>[10x]SVDREEMIERFANFLREYTDEDGNPVYRGKITDLLTITPKRSVAIDWMHLNSFDSELAHEVIENPEEGISAAEDAIQIVLREDFQREDVGKIHARFYNLPETLMVKDIGAEHINKLIQVEGIVTRVGEIKPFVSVAVFVCKDCGHEMIVPQKPYESLEKVKKCEQCGSKNIELDVNKSSAVNFQSFRIQDRPETLKGGEMPRFIDGILLDDIVDVALPGDRVIVTGILRVVLEKREKTPIFRKILEVNHIEPVSKEI

The Minichromosome Maintenance (MCM) complex forms an essential hexameric-ring helicase that unwinds DNA at the replication fork (1–3). MCM proteins have three conserved domains: an N-terminal domain (MCMN) that mediates the head-to-head interaction of the initial double-hexamer; a conserved AAA+ ATPase domain; and a short helix-turn-helix domain at the C-terminus. Crystal structures of the N-terminal domains of Methanobacterium thermautotrophicus (MtMCMN), Sulfolobus solfataricus (SsoMCMN) and Pyrococcus furiosis (PfMCMN) show a consistent hexameric ring structure with three subdomains: a helical subdomain-A, a Zn-binding subdomain-B and an OB-fold subdomain-C. The crystal structure of PfMCMN bound to single-stranded DNA (ssDNA) revealed that subdomain-C binds ssDNA in the plane of the hexameric ring via conserved residues defined as the MCM single-stranded DNA-binding motif (MSSB).

The second mutant (PfMCMN-F179A) involves a residue at the heart of an inter-subunit hydrophobic interface in the PfMCMN-WT hexamer crystal structure. This phenylalanine aligns in sequence with a phenylalanine of Mcm4 whose mutation, Mcm4(Chaos3), severely disrupts Mcm4:Mcm6 association and has been associated mammary adenocarcinoma. The crystal structure of PfMCMN-F179A is isomorphic with that of PfMCMN-βT and shows a similar central pentamer with adjacent subunits interacting via a short antiparallel β-sheet interaction: P130 carbonyl - F240 amide and V132 amide - P238 carbonyl with a shift in the P238 carbonyl position relative to PfMCMN-WT that is similar to PfMCMN-βT. The shifted positions of the P238 carbonyl and the β-turn are likely not directly induced by the F179A mutation because this mutation is not in close proximity. Instead, this structure suggests that the wild-type β-turn can be induced to accommodate either pentameric or hexameric ring structures. AUC sedimentation velocity experiments of PfMCMN-F179A (470 μM) and PfMCMN-ΔZFD (360 μM) showed exclusively monomeric species at all concentrations tested, indicating that these mutants do not form detectable oligomers in solution. The pentameric ring structure of PfMCMN-F179A observed crystallaographically is not maintained in solution under all conditions tested. The PfMCMN-F179A pentamer found in the crystal structure is likely stabilized by crystal-packing interactions, including interactions with the peripheral subunits. We therefore consider a ssDNA-bound monomer of PfMCMN-F179A to be the most likely species detected by EMSA at high concentration. The monomeric preference of PfMCMN-F179A is consistent with the ablation of Mcm4:Mcm6 association in MmMcm4 F345I and also the monomer observed by size-exclusion chromatography for the similarly positioned L189D/D191R double-mutant of SsoMCM.> HMQEAERASASDFKNHQLPLARIKKIMKADEDVRMISAEAPVLFAKACEL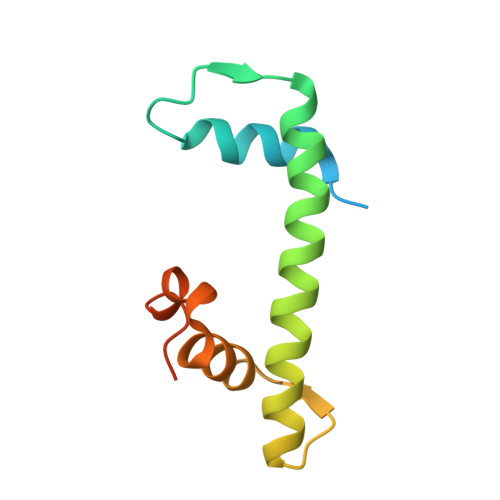FILELTIRSWLHAEENKRRTLQRNDVAAAIARTDVFDFLVDIVPREEAKEEPGS> GAGEARLEEAVNRWVLKFYFHEALRAFRGSRYGDFRQIRDIMQALLVRPLGKEHTVSRLLRVMQCLSRIEEGENLDCSFDMEAELTPLESAINVLEMIKTEFTLTEAVVESSRKLVKEAAVIICIKNKEFEKASKILKKHMSKDPTTQKLRNDLLNIIREKNLAHPVIQNFSYETFQQKMLRFLESHLDDAEPY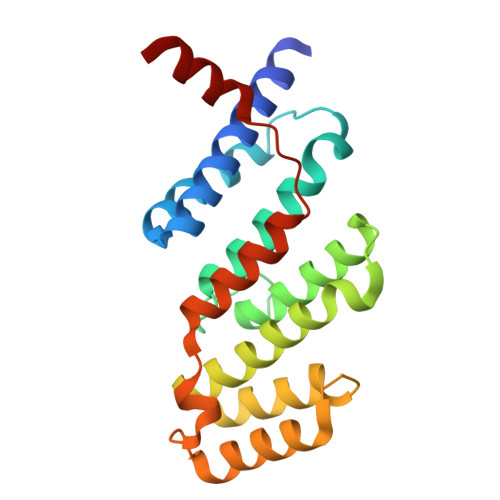LLTMAKKALK Protein lysine methyltransferases (PKMTs) comprise a subfamily of posttranslational modifying enzymes that transfer a methyl group from the cofactor S-adenosyl-L-methionine (SAM). SETD8 (SET8/Pr-SET7/KMT5A) is the sole PKMT annotated for monomethylation of histone H4 lysine 20 (H4K20me) and many nonhistone targets such as the tumor suppressor p53 and the p53-stabilizing factor Numb. Disruption of endogenous SETD8 leads to cell cycle arrest and chromatin decondensation, consistent with essential roles for SETD8 in transcriptional regulation and DNA damage response. Here we solved four distinct crystal structures of SETD8 in alternative ligand-binding states with covalent SETD8 inhibitors and native ligands.

Strikingly, BC-SAM and APO differ from TC by their distinct SET-I motifs in the context of the otherwise similar SET-domain. Furthermore, the post-SET motif of APO structurally resembles an intermediate state between BC-Inh1 and BC-Inh2 but is distinct from those of BC-SAM and TC. In contrast to the structurally diverse SET-I (I1-3) and post-SET motifs (P1-4) in these structures, their pre-SET motifs show only slightly altered configuration. The differences between these structures highlight the conformational plasticity of the SET-I and post-SET motifs. The BC-SAM, BC-Inh1, BC-Inh2, APO, and TC structures can be readily classified into three distinct SET-I configurations (I1-3) and four distinct post-SET configurations (P1-4). Interconversions between metastable conformers cover a broad spatio-temporal scale in particular associated with motions of SETD8’s SET-I and post-SET motifs. In the apo landscape, the general structural features of the X-ray structures of BC-Inh1, BC-Inh2, APO, BC-SAM and TC are recapitulated by a subset of macrostates (e.g. A6 for BC-Inh1; A10 for BC-Inh2; A12 for APO; A20 for BC-SAM; A22, A24 for TC, 6 of 24 macrostates, Figure 11).

> GGSSRKSKAELQSEERKRIDELIESGKEEGMKIDLIDGKGRGVIATKQFSRGDFVVEYHGDLIEITDAAARAALYAQDPSTGCYMYYFQYLSKTYCVDATRETNRLGRLINHSKCGNCQTKLHDIDGVPHLILIASRDIAAGEELLYDYGDRSKASIEAHPWLKH> RDYDHLFKLLIIGDSGVGKSSLLLRFADNTFSGSYITT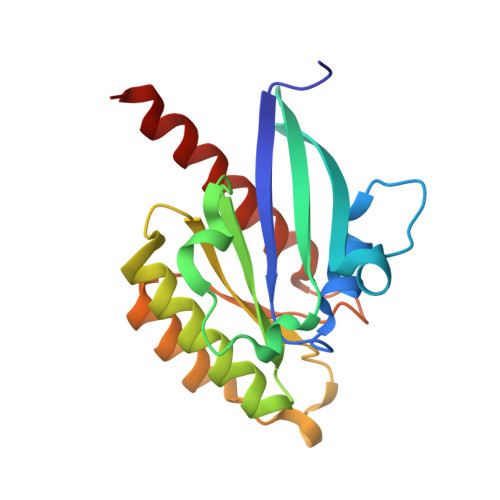IGVDFKIRTVEINGEKVKLQIWDTAGQERFRTITSTYYRGTHGVIVVYDVTSAESFVNVKRWLHEINQNCDDVCRILVGNKNDDPERKVVETEDAYKFAGQMGIQLFETSAKENVNVEEMFNCITELVLRAKKDNLAK> GPMEQLKCCSGILKEMFAKKHAAYAWPFYKPVDVEALGLHDYCDIIKHPMDMSTIK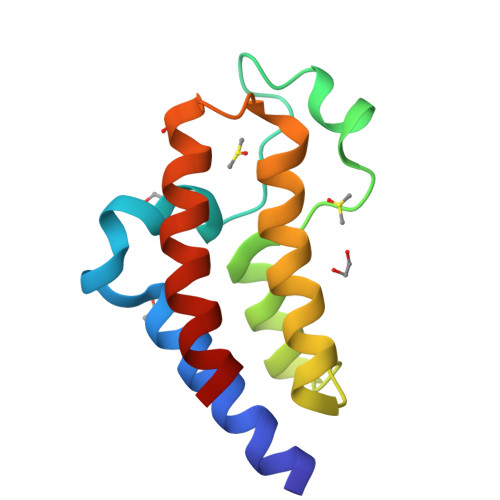SKLEAREYRDAQEFGADVRLMFSNCYKYNPPDHEVVAMARKLQDVFEMRFAKM> TLPAVISRWLSSVLPGGAAPEVTVESGVDSTGMSSETIILTARW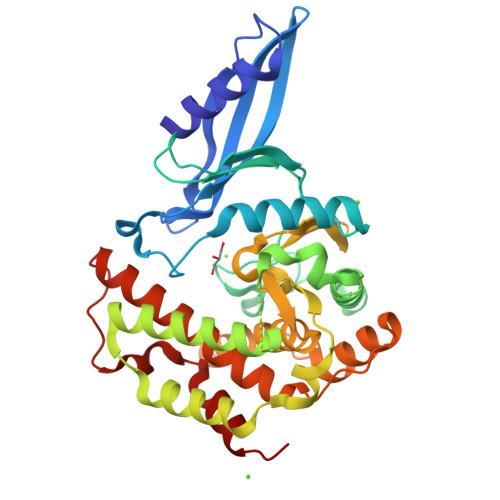QQDGRSIQQKLVARVAPAAEDVPVFPTYRLDHQFEVIRLVGELTDVPVPRVRWIETTGDVLGTPFFLMDYVEGVVPPDVMPYTFGDNWFADAPAERQRQLQDATVAALATLHSIPNAQNTFSFLTQGRTSDTTLHRHFNWVRSWYDFAVEGIGRSPLLERTFEWLQSHWPDDAAAREPVLLWGDARVGNVLYRDFQPVAVLDWEMVALGPRELDVAWMIFAHRVFQELAGLATLPGLPEVMREDDVRATYQALTGVELGDLHWFYVYSGVMWACVFMRTGARRVHFGEIEKPDDVESLFYHAGLMKHLLGEEH OCTANE 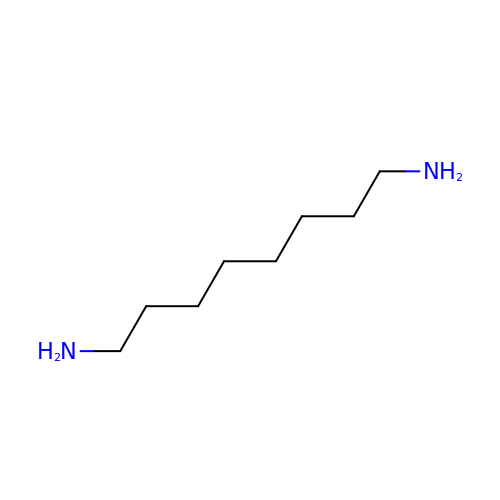1,8-DIAMINE | C8 H20 N2 | PWGJDPKCLMLPJW-UHFFFAOYSA-N(2S,3S)-3-HYDROXYARGININE | C6 H14 N4 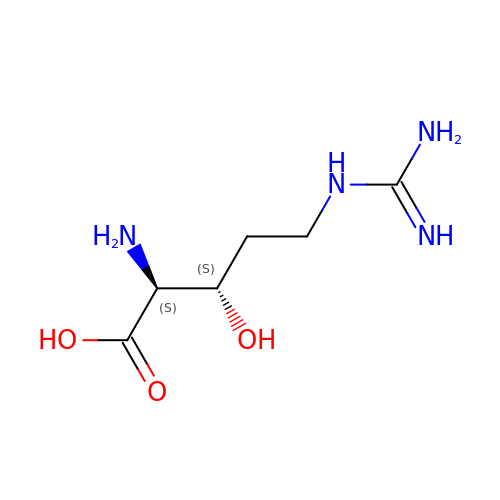O3 | VIDUVSPOWYVZIC-IMJSIDKUSA-N> RPPLQEYVRKLLYKDLSKVTTEKVLRQMRKLPWQDQEVKDYVICCMINIWNVKYNSIHCVANLLAGLVLYQE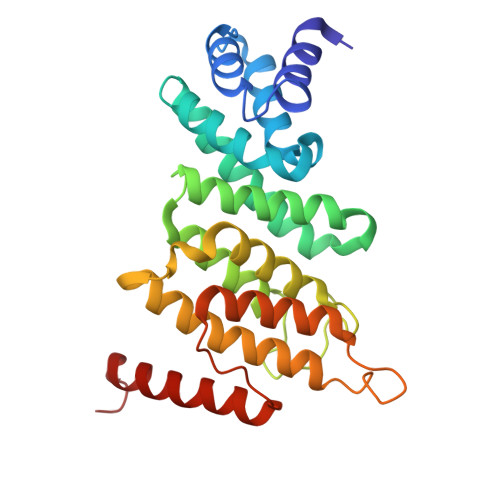DVGIHVVDGVLEDIRLGMEVNQPKFNQRRISSAKFLGELYNYRMVESAVIFRTLYSFTSFGVNPDGSPSSLDPPEHLFRIRLVCTILDTCGQYFDRGSSKRKLDCFLVYFQRYVWWKKSLEVWTKDHPFPIDIDYMISDTLELLRPKIKLCNSLEESIRQVQDLEREFLIKLGLVN> MGSSHHHHHHENLYFQGHMENPANANPIRVGVIGCADIAWRRALPALEAEPLTEVTAIASRRWDRAKRFTERFGGEPVEGYP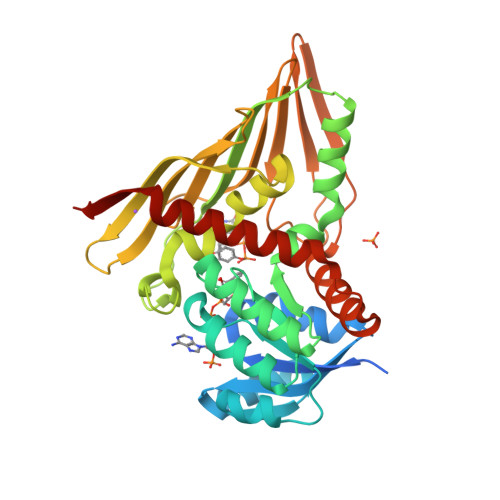ALLERDDVDAVYVPLPAVLHAEWIDRALRAGKHVLAEKPLTTDRPQAERLFAVARERGLLLMENFMFLHHPQHRQVADMLDEGVIGEIRSFAASFTIPPKPQGDIRYQADVGGGALLDIGVFPIRAAGLFLGADLEFVGAVLRHERDRDVVVGGNALLTTRQGVTAQLTFGMEHAYTNNYEFRGSTGRLWMNRVFTPPATYQPVVHIERQDHAEQFVLPAHDQFAKSIRAFAQAVLSGEHPREWSEDSLRQASLVDAVRTGARDIYFP> MDAKQRIARRVAQELRDGDIVNLGIGLPTMVANYLPEGIHITLQSENGFLGLGPVTTAHPDLVNAG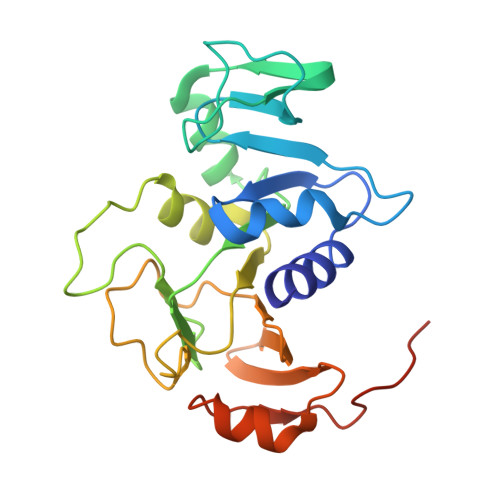GQPCGVLPGAAMFDSAMSFALIRGGHIDACVLGGLQVDEEANLANWVVPGKMVPGMGGAMDLVTGSRKVIIAMEHCAKDGSAKILRRCTMPLTAQHAVHMLVTELAVFRFIDGKMWLTEIADGCDLATVRAKTEARFEVAADLNTQRGDLTHHHHHH The CP folds into three jelly-roll β sandwiches. The B and C domains clustered at the 3-fold axis. The structural variability of CP subunits within a capsid was very low. GFLV and TRSV are both transmitted by Xiphinema nematodes.

differs from its parent strain (GFLV-F13) by a single Gly297Asp mutation. position 297 is replaced by Asp. deficiency of GFLV-TD by X. index. transmission was correlated with a lack of virus retention by X. index, although virus acquisition by nematodes was not affected. solvation shell via the addition of 60 negative charges in GFLV-TD. with respect to that of wild-type GFLV-F13. feeding apparatus, thereby reducing its transmissibility. ligand-binding pocket was correlated to a defect in virus transmission.

>[20x]GLAGRGVIYIPKDCQANRYLGTLNIRDMISDFKGVQYEKWITAGLVMPTFKIVIRLPANAFTGLTWVMSFDAYNRITSRITASADPVYTLSVPHWLIHHKLGTFSCEIDYGELCGHAMWFKSTTFESPRLHFTCLTGNNKELAADWQAVVELYAELEEATSFLGKPTLVFDPGVFNGKFQFLTCPPIFFDLTAVTALRSAGLTLGQVPMVGTTKVYNLNSTLVSCVLGMGGTVRGRVHICAPIFYSIVLWVVSEWNGTTMDWNELFKYPGVYVEEDGSFEVKIRSPYHRTPARLLADQSQRDMSSLNFYAIAGPIAPSGETAQLPIVVQIDEIVRPDLSLPSFEDDYFVWVDFSEFTLDKEEIEIGSRFFDFTSNTCRVSMGENPFAAMIACHGLHSGVLDLKLQWSLNTEFGKSSGSVTITKLVGDKAMGLDGPSHVFAIQKLEGTTELLVGNFAGANPNTRFSLYSRWMAIKLDQAKSIKVLRVLCKPRPGFSFYGRTSFPV>[2x]GMAQGLIEVERKFAPGPDTEERLQELGATLEHRVTFRDTYYDTSELSLMLSDHWLRQREGSGWELKCPGVTGVSGPHNEYVEVTSEAAIVAQLFE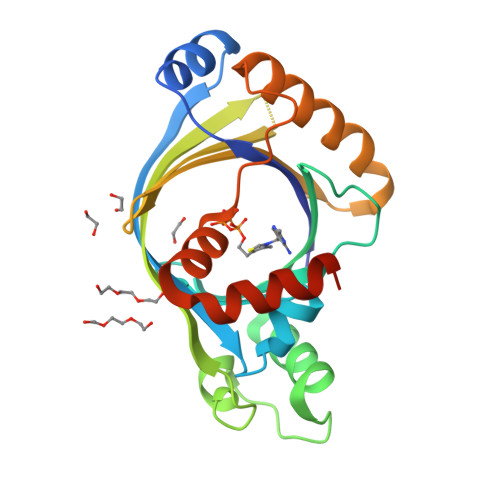LLGSGEQKPAGVAAVLGSLKLQEVASFITTRSSWKLALSGAHGQEPQLTIDLDSADFGYAVGEVEAMVHEKAEVPAALEKIITVSSMLGVPAQEEAPAKLMVYLQRFRPLDYQRLLEAASSGEATGDSASS>GPGSMVSDLVQVERNGPVTTVIINRPQARNAVNGPTAAALYSAFAEFDRDESASVAVLCGNGGTFCAGADLKAFGTAEANAVHRTGPGPMGPSRMMLSKPVIAAVSGYAVAGGLELALWCDLRVAEQDAVFGVFCRRWGVPLIDGGTVRLPRLIGHSRAMDMILTGRAVQ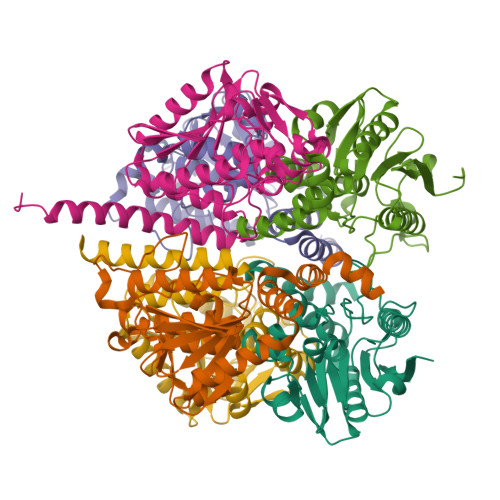ADEALAIGLANRVVPNGQARQAAEELAAQLAALPQQCLRSDRLSALQQWGLPESAALDLEFASISRVAAEALEGAGRFAAGAGRHGAQASH[6x]>MKVAVLPGDGIGPEVTEAALKVLRALDEAEGLGLAYEVFPFGGAAIDAFGEPFPEPTRKGVEEAEAVLLGSVGGPKWDGLPRKIRPETGLLSL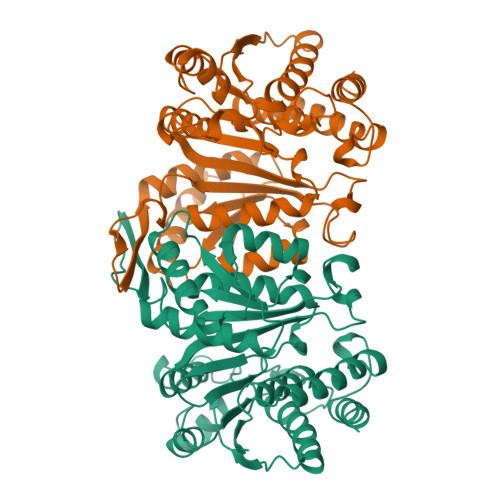RKSQDLFANLRPAKVFPGLERLSPLKEEIARGVDVLIVRELTGGIYFGEPRGMSEAEAWNTERYSKPEVERVARVAFEAARKRRKHVVSVDKANVLEVGEFWRKTVEEVGRGYPDVALEHQYVDAMAMHLVRSPARFDVVVTGNIFGDILSDLASVLPGSLGLLPSASLGRGTPVFEPVHGSAPDIAGKGIANPTAAILSAAMMLEHAFGLVELARKVEDAVAKALLETPPPDLGGSAGTEAFTATVLRHLA[4x]> NDINKIELKNLSGEIIKENGKEAIKYTSSDTASHKGWKATLSGTFIEDPHSDKKTALLNLEGFIPSDKQIFGSKYYGKMKWPETYRINV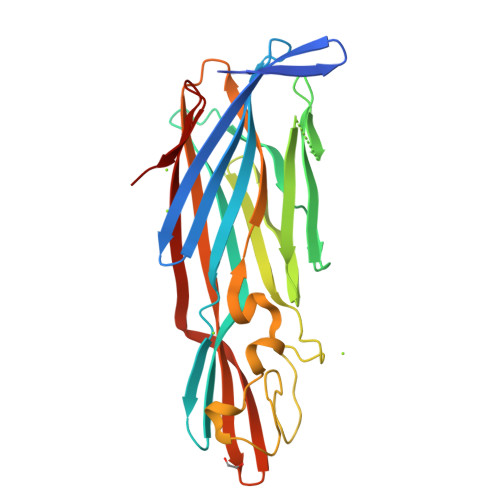KSADVNNNIKIANSIPKNTIDKKDVSNSIGYSIGGNISVEGKTAGAGINASYNVQNTISYEQPDFRTIQRKDDANLASWDIKFVETKDGYNIDSYHAIYGNQLFMKSRLYNNGDKNFTDDRDLSTLISGGFSPNMALALTAPKNAKESVIIVEYQRFDNDYILNWETTQWRGTNKLSSTSEYNEFMFKINWQDHKIEYYL> MGYYEDDRETIEISESRVSRGSSRGPRSRGGDYAPNTVSIPCHHIRLGDILLLQGRPCQVIRISTSAATGQHRYLGVDLFTKELREESSSISTPSPSVVVQTMCGPVFKQYRVLDMQAG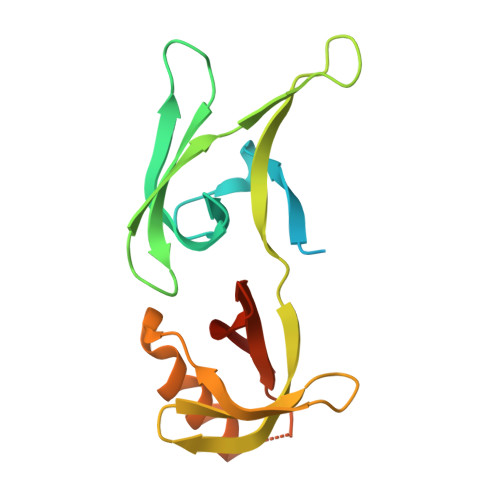HIVAMTETGDVKQNLPVSEQSNLYERLQRAFESGRGSVRALVVSDNGRELVCDMAVLHGSRL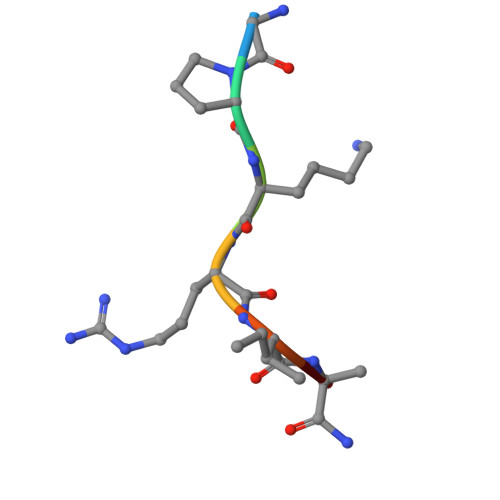> GPKRIAX>GMAEPNGQSAPNGTTSNGRPSYAEKHKLPAHFIGGNRLENAPPSKVKDFVAEHGGHTVITNVLIANNGIAAVKEIRSVRKWAYETFGDERAIKFTVMATPEDLQANADYIRMADHYVEVPGGTNNHNYANVELIVDVAERMDVHAVWAGWGHASENPKLPESLAASPKKIVFIGPPGSAMRSLGDKISSTIVAQHANVPTIPWSGSGVSEVHIDENGIVTVPEEVYLKGCVNSWEEGLEKAREIGFPVMIKASEGGGGKGIRKCMNEDQFEELYKAAAAEIPGSPIFIMKLADSARHLEVQLLADQYGNNISLFGRDCSVQRRHQKIIEEAPVTIASPTTFRAMEEAAVRLGKLVGYVSAGTVEYLYSHADDKFYFLELNPRLQVEHPTTEMVSGVNLPAAQLQIAMGIPLHRIRDIRLLYGVDPKAATEIDFEFKNPESEKTQRRPAPKGHTTACRITSEDPGEGFKPSSGMLQELNFRSSSNVWGYFSVGTAGGIHSFSDSQFGHIFAYGENRAASRKHMIVALKELSIRGDFRTTVEYLIKLLETQAFEENTITTGWLDELISKKLTAERPDTNLAIICGAVIRAHTESEKSLADYRAGLEKGQVPSKDILKTVSSVDFIYEGLRYKFTVTRSSVDTYRLFINGSQCEVGVRTLSDGGLLVLLGGHSHNVYWKDEATGTRISIDGKTCLLEQENDPTGSGALDDPSRVKQAQPFVGQLPQYGSPVVVGSKPAQRFAVLYGTMCDILNGYDNQVVMQQKLKEFIEVLRDPKLPYSEFSAQFSALHARMPHKLDAQLTQVLERAQNRGAEFPARQLLKVFNKFLDDNVPNKTDQDLLKSTLEPLTSVLNLYLDGQKARELNLIADLLSMYADVECQFSGRRLQDEEAILKLRDQYKDNIQKVVNTVLSHKNVMSKNSLVLALLDEYRPNKPNVGNVGKHLRPVLRRLTELESRQSAKVSLKAREVLILCALPSLEERTAQMEHILRSSVVQSRYGETGWSHRRPDREVLKEVVDSKYTVFDVLTLFFAHEDPYVALAALEVYVRRAYRAYNLREVRYHDEERPYFIDWDFALRKSGANQTESSMHMQSVVPSSPATPVENDFKRIHSISDMTYLARRTRDEPIRKGVIVPCKDLLDAEEALSRALEVLPLAHKETKDKDRKQQPGIAADLAQRRRPGTPLRLEGIGELSAVVNVAVRDAEGKNDEEILALIKPWVQNSKADLLARRVRRLTFICGRNDGSYPSYYTFRGPDYAEDDSIRHIEPSLAFQLELGRLSKFKLTPVFTQNKNIHVYEAVGRGVETDRRYFTRAVVRPGRLRDEISTAEYLISEADRVVNDIFDALEIIGTNKTDLNHMFINFSHTFQVTADEVAESLQGFLDRFGPRGWRLRVHQVEIRINCMRSDNNDENDTMPLRVIITNTSGFVIQIELYEEKLSEKGEWVYYYVSGNAKIGSMHLLPVSTPYPTKNWLQPKRYKAHILGTQYVYDFPELFRQAIQNSWTEAVKKIPSLAAKQPAIGECIDYNELVLGDQDNLAEVSREPGMNSTG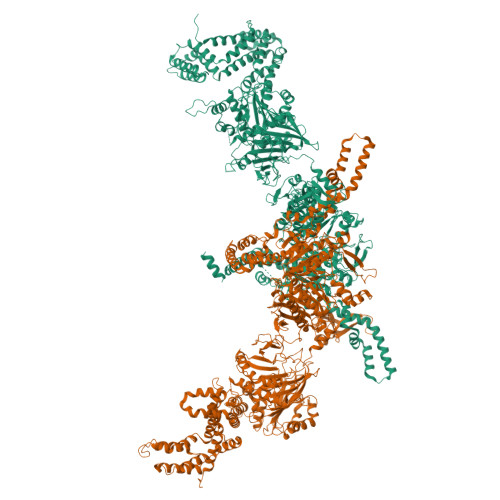MVGWLINARTPEYPDGRKFIVVANDITFKIGSFGPKEDTFFFKCTELARKMGIPRIYLSANSGARLGLAEELMPHFNVAWNDPAKPEAGFKYLYLSDEAKRRFENEVITEEIVEDGEKRHKIITIVGAEEGLGVECLRGSGLIAGATSRAYNDIFTCTLVTCRSVGIGAYLVRLGQRAVQVEGQPIILTGAPALNSLLGREVYTSNLQLGGTQIMYRNGVSHLTAKDDFDGVTKIVQWLSFIPDQRNNPLPILSPSPDPWDRDVVYTPPYKQTYDVRWMIAGKEDEDGFQPGLFDKDSFVETLGGWARTVVVGRARLGGIPMGVIAVETRTIENITPADPANPDSIEQVTNEAGGVWYPNSAFKTAQAINDFNYGEQLPLMILANWRGFSGGQRDMYNEVLKYGSFIVDALTRFEKPIFIYIPPHGELRGGSWVVVDPTINPASMEMYADEEARGGVLEPEGIIPIKYKKDKQLETMARLDPVYRSLKKEMAKEGLSKEESDNIKKKMQQREELLLPIYHQICVQFADLHDRAGRMKAKGVIRQSLQWRQSRRFFYWRVRRRLIEDDILRRIEEAINPAGKRRHDPENTSLAASPETRSPHLVQLESWVGIPGFKTNDREVVEWYEQNQDRINEKLEKLKKESIADQMRELLRXXXXXXXXXXXX[2x]>[3x]MGETKVIYHLDEEETPDLVKIPVPAERITLGDFKSVLQRPAGAKYFFKSMDQDFGVVKEEISDDNARLPCFNGRVVSWLVSSDNPQPEMAPPVHEPR

Dvl is a pivotal factor in Wnt signal transduction, relaying Wnt signals to canonical and non-canonical downstream effectors. It contains three domains (separated by long flexible linkers) through which it binds to its signalling partners, typically with weak affinity. These weak interactions depend on dynamic and concentration-dependent polymerization by the DIX domain5, which transiently generates high local concentrations of binding sites. Signalosome formation by Dvl depends on head-to-tail polymerization by its DIX domain56, which also hetero-polymerizes with the DIX domain of Axin7, thereby recruiting Axin degradasomes to the plasma membrane.

To understand the structural basis for the polymerization block imposed by DIX54-Ub, we purified the hDvl2 DIX domain (bearing Y27D), and solved its crystal structure at 2.7 Å resolution. Like other DIX domains5, the hDvl2 DIX monomer exhibits a ubiquitin-like fold, with five β-strands and an α-helix. Its structure is very similar to that of the Dvl1 DIX monomer11 (with a root-mean-square deviation (r.m.s.d). for the core Cα backbone of 1.14 Å between hDvl2 MolA and Dvl1 MolF), whereby the main differences are in two loop regions (between β1 and β2, and α1 and β3). There are marked differences in the dimensions of the DIX filament structures in the crystals: the filament of hDvl2 DIX is ∼67 Å wide, and its repeat length is 85 Å, with 6 monomers per turn, almost identical to the Axin DIX filament, whereas the filament in the Dvl1 DIX domain crystal (from the equivalent mutant, Y17D) is nearly twice as long as the Axin DIX filament, with a repeat length of ∼140 Å and 8 monomers per turn. As the helical pitch determines the packing of adjacent filaments in the crystals, it is unsurprising that the two types of DIX filaments contact each other at different sites (termed site III), but it seems likely that these contacts, like the filamental dimensions, simply reflect the different crystallization conditions. hDvl2 K54 and K58 are both located within the DIX tail portion: K54 lies at the junction between β3 and the preceding loop, flanking the DIX–DIX interface and pointing towards this interface (roughly parallel to the M2 residue V67), whereas K58 is within β3, but points away from this interface into the solvent. This predicts that a Ub moiety attached to K54 would create a steric clash with the head surface of an interacting DIX monomer, whereas one attached to K58 would be oriented perpendicularly to the filamental axis and thus not impinge on the DIX–DIX interaction (although we note that ubiquitin contains an extended flexible C-terminus, and may thus be able to adopt multiple conformations relative to the DIX domain). Given that K58 projects into the inside of the helical filament, stoichiometric ubiquitination of this residue might affect the filamental shape, which could explain why this modification limits oligomerization to a single helical pitch in solution.One of the best-studied LEM-domain proteins is emerin, a ubiquitously-expressed integral protein anchored at the nuclear membrane. It consists of 254 amino acids including an N-terminal LEM-domain, a large intrinsically disordered region (IDR) and a short transmembrane segment. The emerin LEM-domain binds to the highly conserved DNA-binding protein barrier-to-autointegration factor (BAF, also known as Banf1). Finally, BAF is able to mediate interaction between emerin and the lamin A/C tail.

Interestingly, missense mutations (P22L, T43I) and a small deletion (ΔK37) associated with exclusive cardiac defects were detected in emerin LEM-domain that interacts with the DNA binding protein BAF. Indeed, this emerin LEM-domain directly interacts with the barrier-to-autointegration factor (BAF), an 89-residue protein that binds to double-stranded DNA. Analysis of the 3D structure of the LEM-BAF complex reveals that emerin Pro22 and Lys37 belonged to a well-conserved surface that is involved in BAF binding (in blue on Figure 3a). By contrast, Thr43 mutation was located on the opposite side of the LEM-domain, far from the interface with BAF. Only a few signals corresponding to the residues close to the site of mutation are shifted, demonstrating that the mutations P22L and T43I do not modify the 3D structure of the emerin construct EmN. Finally, we tried to crystallize the ternary complexes formed by the EmN mutants, BAF and the Igfold domain of lamin A/C using the same protocol used for wild-type EmN. We succeeded in solving the 3D structure of the complex containing EmN T43I at a resolution of 2.3 Å. The structure of the mutated LEM-domain bound to the BAF dimer is displayed on Figure 3c. Analysis of the crystal structure of EmN T43I bound to BAF corroborated that this mutation does not perturb the interface with BAF.

> FSQHARTSGRVAVEEVDEEGKFVRLRNKSNEDQSMGNWQIKRQNGDDPLLTYRFPPKFTLKAGQVVTIWAAGAGATHSPPTDLVWKAQNTWGCGNSLRTALINSTGEEVAMRKLVR;>TSQKHRDFVAEPMGEKPVGSLAGIGEVLGKKLEERGFDKAYVVLGQFLVLKKDEDLFREWLKDTAGANAKQSRDAFGALREWADAFL[2x];> DNYADLSDTELTTLLRRYNIPHGPVVGSTRRLYEKKIFEYEIQ3-{[(4-cyanophenyl)methyl](1-oxo-1,2-dihydroisoquinolin-7-yl)sulfamoyl}benzene-1-sulfonyl fluoride | C23 H16 F N3 O5 S2 | 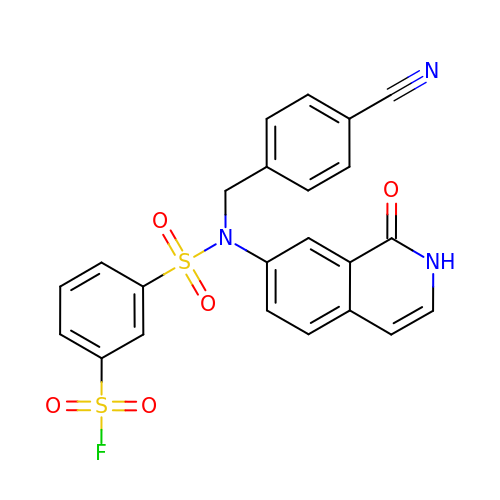VDEDGNULGMBOAN-UHFFFAOYSA-N> FSIAVTGATGQLGGLVIQHLMAAVPASQIIAIVRNVEKASTLADQGVEVRHGDYNQPESLQKAFAGVSKLLFISGPHYDNTLLIVQHANVVKAARDAGVKHIAYTGYAFAEESIIPLAHVHLATEYATRTTNIPYTFLRNALYTDFFVNEGLRASTESGAIVTNAGSGIVNSVTRNELALAAATVLTEEGHENKTYNLVSNQPWTFDELAQILSEVSGKK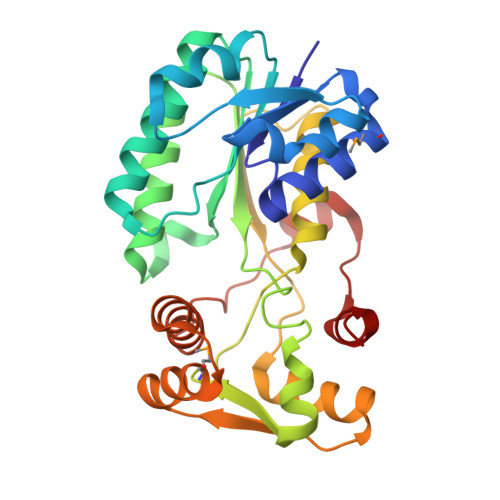VVHQPVSFEEEKNFMVNAGVPEPFAEITAAIYDAISKGEASKTSDDLQKLIGSLTPLKETVKQALKM> DEEGGGEEDQDFDL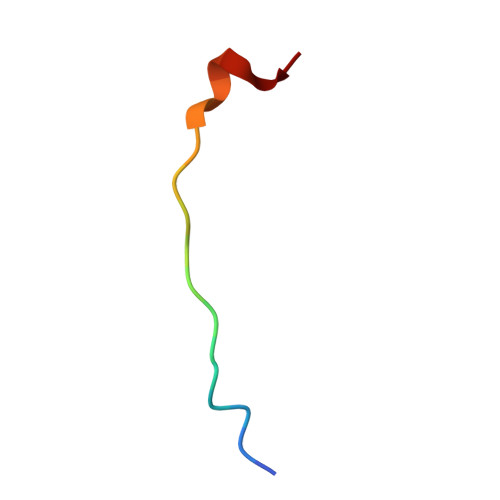SQLH> MANLSGYNFAYLDEQ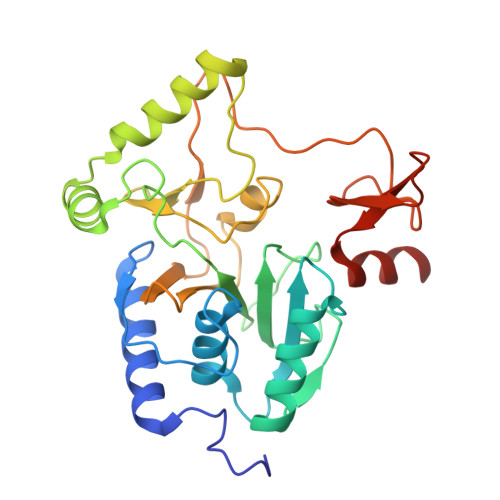TKRMIRRAILKAVAIPGYQVPFGGREMPMPYGWGTGGIQLTASVIGESDVLKVIDQGADDTTNAVSIRNFFKRVTGVNTTERTDDATVIQTRHRIPETPLTEDQIIIFQVPIPEPLRFIEPRETETRTMHALEEYGVMQVKLYEDIARFGHIATTYAYPVKVNGRYVMDPSPIPKFDNPKMDMMPALQLFGAGREKRIYAVPPFTRVESLDFDDHPFTVQQWDEPCAICGSTHSYLDEVVLDDAGNRMFVCSDTDYCRQQSEAKNQ> GPPGPPGPPGP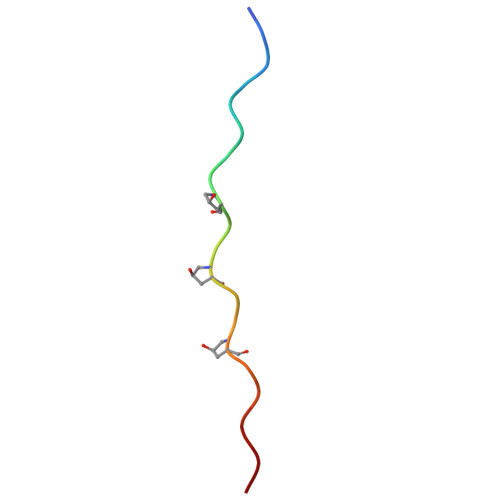PGPPGPPGPP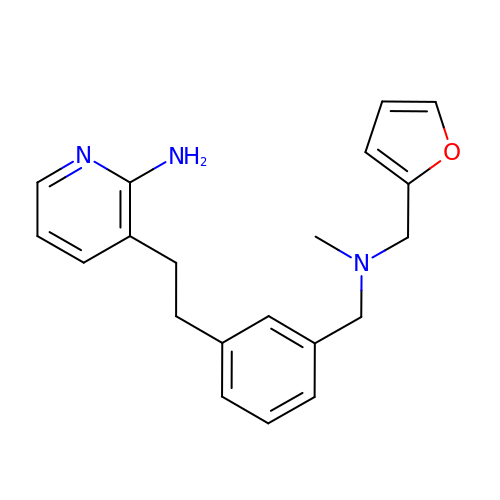3-[2-(3-{[(furan-2-ylmethyl)(methyl)amino]methyl}phenyl)ethyl]pyridin-2-amine | C20 H23 N3 O | PGBSGPMEMSPFFE-UHFFFAOYSA-N>MASLLKVDQEVKLKVDSFRERITSEAEDLVANFFPKKLLELDSFLKEPILNIHDLTQIHSDMNLPVPDPILLTNSHDGLDGPTYKKRRLDECEEAFQGTKVFVMPNGMLKSNQQLVDIIEKVKPEIRLLIEKCNTVKMWVQLLIPRIEDGNNFGV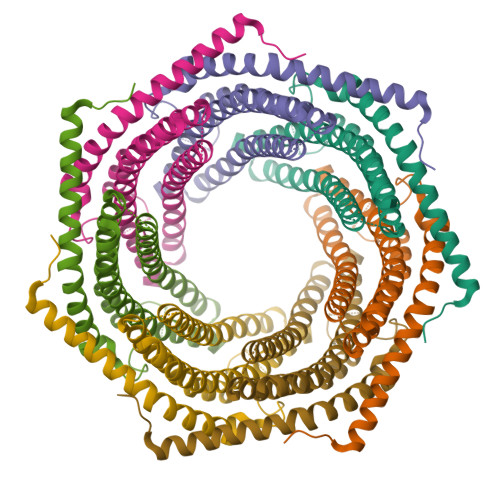SIQEETVAELRTVESEAASYLDQISRYYITRAKLVSKIAKYPHVEDYRRTVTEIDEKEYISLRLIISELRNQYVTLHDMILKNIEKIKRPRSSNAETLY[7x]> MAQTPAFNKPKVELHVHLDGAIKPETILYFGKKRGIALPADTVEELRNIIGMDKPLSLPGFLAKFDYYMPVIAGCREAIKRIAYEFVEMKAKEGVVYVEVRYSPHLLANSKVDPMPWNQTEGDVTPDDVVDLVNQGLQEGEQAFGIKVRSILCCMRHQPSWSLEVLELCKKYNQKTVVAMDLAGDETIEGSSLFPGHVEAYEGAVKNGIHRTVHAGEVGSPEVVREAVDILKTERVGHGYHTIEDEALYNRLLKENMHFEVCPWSSYLTGAWDPKTTHAVVRFKNDKANYSLNTDDPL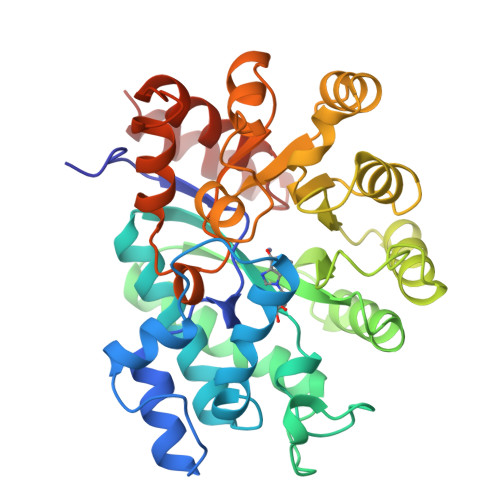IFKSTLDTDYQMTKKDMGFTEEEFKRLNINAAKSSFLPEEEKKELLERLYREYQ> SNAMGKTNNILYVMSGQNFQDEEYFESKKIFESAGYKTKVSSTFIGTAQGKL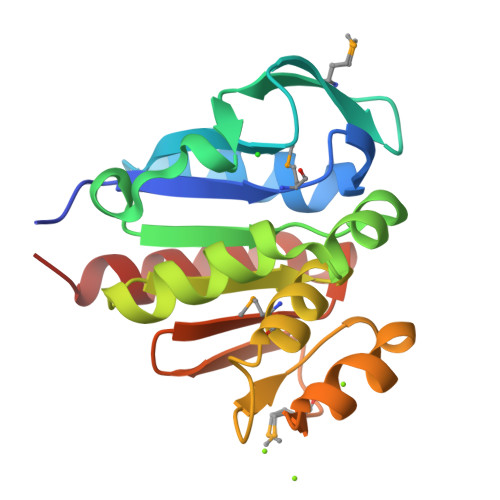GGMTNIDLLFSEVDAVEFDAVVFVGGIGCITLWDDWRTQGLAKLFLDNQKIVAGIGSGVVIMANAKILEEINVTCLSADESHVRHGNANIMSENVVVSGNIVTANGPTSSKDFANAVVGVLNSLS>SMGAGGGGSAEQLDALVKKDKVVVFLKGTPEQPQCGFSNAVVQILRLHGVRDYAAYNVLDDPELRQGIKDYSNWPTIPQV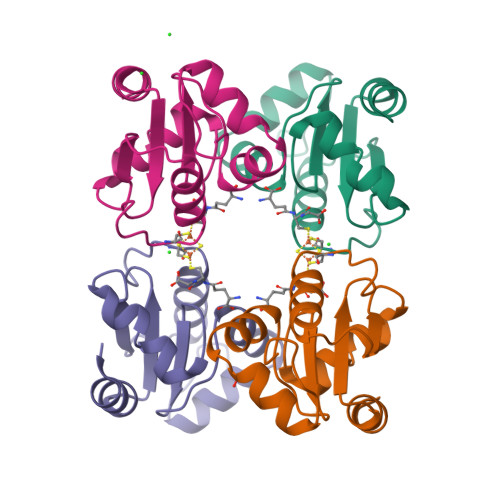YLNGEFVGGCDILLQMHQNGDLVEELKKLGIHSALLDE[4x]> GSHMEAVQNRIVEAAERVPGVRGVIHLRARYVGQDIWADMIIGVDPENTVEQAAEISEAVQAA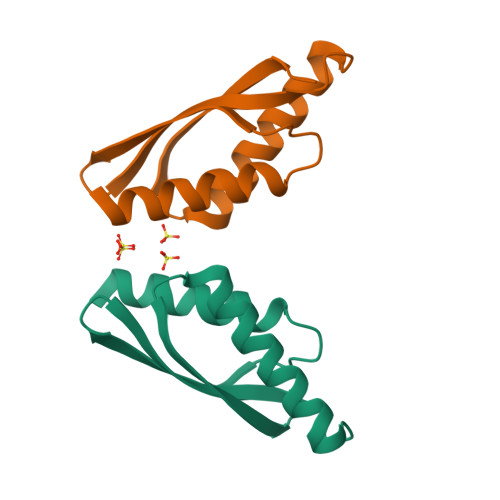VCGKIRRIESLHVSAAAREIGDTTKPSFSDQPLSFDEVMLSKVDN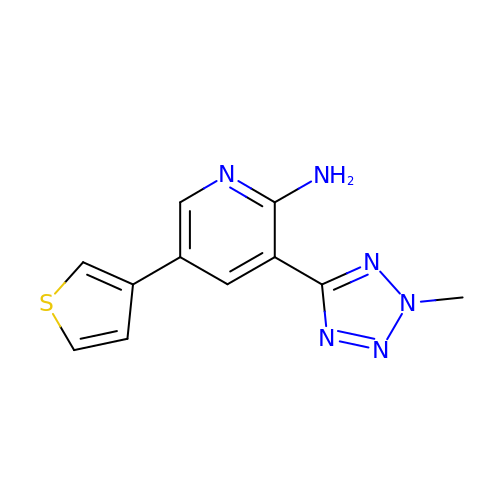3-(2-methyltetrazol-5-yl)-5-(3-thienyl)pyridin-2-amine | C11 H10 N6 S | SYTWVNLAKXLKOD-UHFFFAOYSA-N2-oxidanylidenepropyl 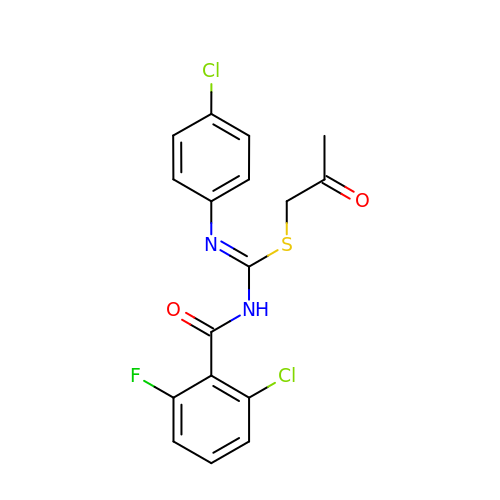~{N}-(2-chloranyl-6-fluoranyl-phenyl)carbonyl-~{N}'-(4-chlorophenyl)carbamimidothioate | C17 H13 Cl2 F N2 O2 S | WKKVCWKOLYDIGO-UHFFFAOYSA-N>MQVIPACNSAAIRSLCPTPESFRNMGWLSVSDAVYSEFIGELATRASNRNYSNEFGLMQPIQEFKAFIESDPVVHQEFIDMFEGIQDSPRNYQELCNMFNDIFRKAPVYGDLGPPVYMIMAKLMNTRAGFSAFTRQRLNLHFKKLFDTWGLFLSSKDSRNVLVADQFDDRHCGWLNERALSAMVKHYNGRAFDEVFLCDKNAPYYGFNSYDDFFNRRFRNRDIDRPVVGGVNNTTLISAACESLSYNVSYDVQSLDTLVFKGETYSLKHLLNNDPFTPQFEHGSILQGFLNVTAYHRWHAPVNGTIVKIINVPGTYFAQAPSTIGDPIPDNDYDPPPYLKSLVYFSNIAARQIMFIEADNKEIGLIFLVFIGMTEISTCE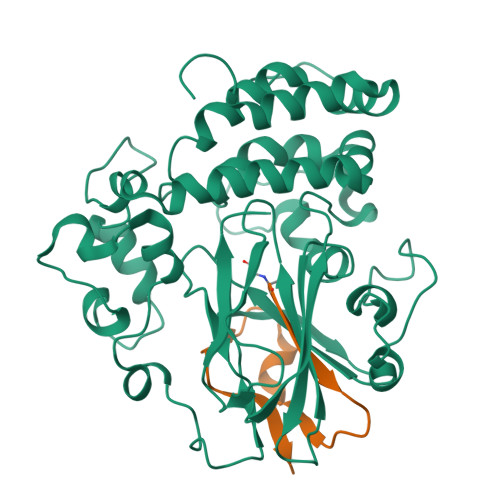ATVSEGQHVNRGDDLGMFHFGG[6x];>[6x]XSFALGLRKDCRAEIVEKFTEPGTVIRINEVVAALKA>MQSLTTALENLLRHLSQEIPATPGIRVIDIPFPLKDAFDALSWLASQQTYPQFYWQQRNGDEEAVVLGAITRFTSLDQAQRFLRQHPEHADLRIWGLNAFDPSQGNLLLPRLEWRRCGGKATLRLTLFSESSLQHDAIQAKEFIATLVSIKPLPGLHLTTTREQHWPDKTGWTQLIELATKTIAEGELDKVVLARATDLHFASPVNAAAMMAASRRLNLNCYHFYMAFDGENAFLGSSPERLWRRRDKALRTEALAGTVANNPDDKQAQQLGEWLMADDKNQRENMLVVEDICQRLQADTQTLDVLPPQVLRLRKVQHLRRCIWTSLNKADDVICLHQLQPTAAVAGLPRDLARQFIARHEPFTREWYAGSAGYLSLQQSEFCVSLRSAKISGNVVRLYAG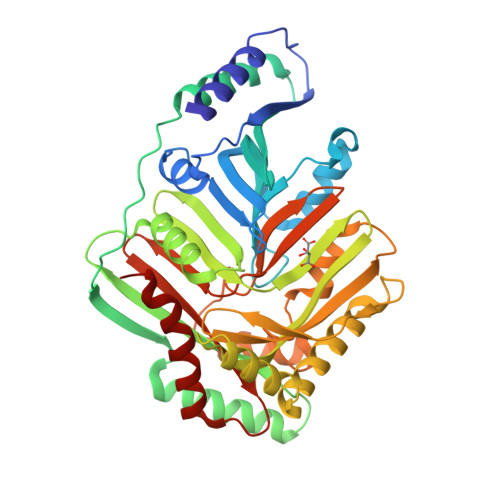AGIVRGSDPEQEWQEIDNKAAGLRTLLQME[2x]>[3x]GSHMGTEDLKYSLERLREILERLEENPSEKQIVEAIRAIVENNAQIVEAIRAIVENNAQIVEILRAIIEALEAIGGGTKILEEMKKLLKDLKRSLERG

We used de novo protein design to generate very closely related proteins that adopt two very different states—a short state and a long state, like a viral fusion protein—and then created a single molecule that can be found in both forms. Inspired by class I viral fusion proteins, such as influenza hemagglutinin, we chose homotrimeric helical bundles as the fundamental architecture. We decided on a design scheme with two divergent conformations containing a constant six-helix bundle “base” and a variable portion with three inner helices and three “flipping” helices. In the compact “short” state (∼66 Å height), the flipping helices fold back to interact with the inner helices; in the extended “long” state (∼100 Å height), they extend to form interactions with each other.

The interaction energy between the flipping helix and the inner helices in the short state was tuned by combining hydrogen bond layers (“A”) or hydrophobic layers (“X”) in different orders in each of three possible positions. Designs were given three-letter names corresponding to the layers in order, starting at the hinge proximal position. We constructed all eight possible permutations of two different layers in three positions, dubbed SERPNTs (in silico engineered rearrangeable protein topologies). The number and position of the hydrogen bond networks appears to determine the state which is populated—designs with one network folding into the short state, with two networks, into a more dynamic short state, and with three networks, into the long state. The hydrogen-bond network residues were closer to the computational model in XAX than in XXA, likely because they were buried in the former and solvent exposed in the latter.>[3x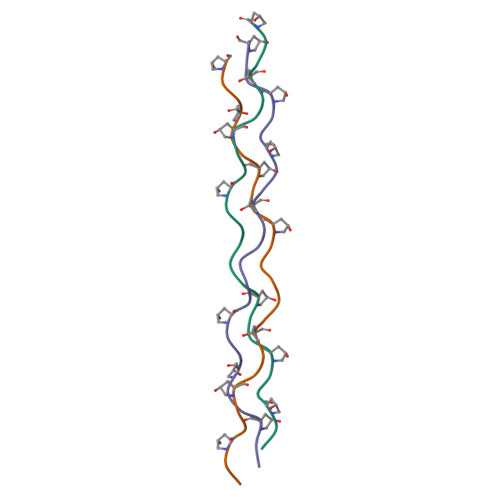]XGPPGPPGPPGPQGFPGPPGPPGPPX> GRPRAINKHEQEQISRLLEKGHPRQQLAIIFGIGVSTLY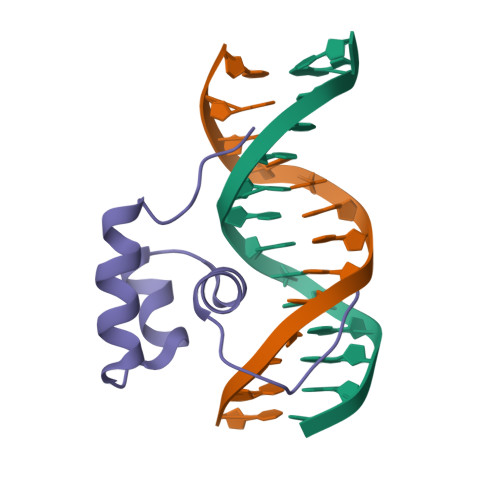RYFPASSIKKRMN> HHHHHHKDEVALLAAVTLLGVLLQAYFSLQVISARQAF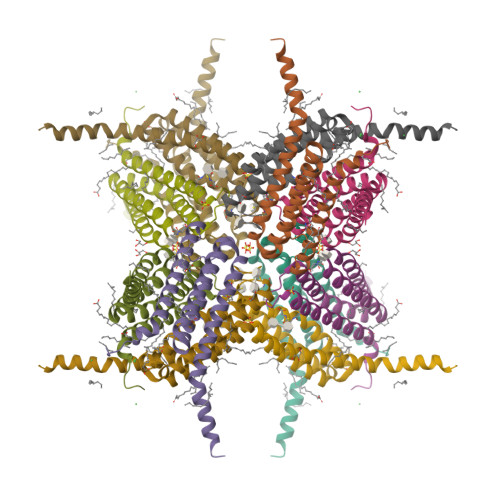RVSPPLTTGPPEFERVYRAQVNCSEYFPLFLATLWVAGIFFHEGAAALCGLVYLFARLRYFQGYARSAQLRLAPLYASARALWLLVALAALGLLAHFLPAALRAALLGRLRTLLPWA> MGNCLDSSAKVDNSNHSPHANSASSGSKVSSKTS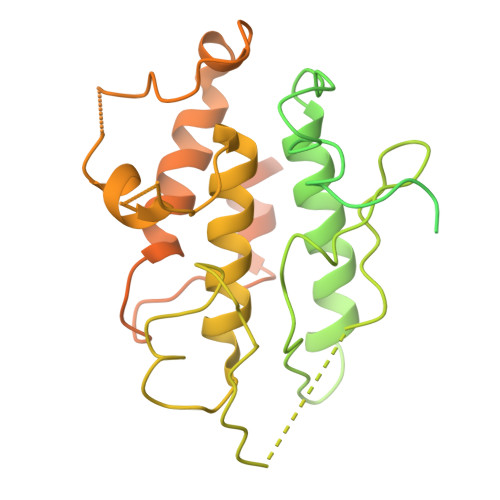RSTGPSGLSTTSYSTDSSFGPLPTLRTEGEILSSPNLKAFTFNELKNATKNFRQDNLLGEGGFGCVFKGWIDQTSLTASRPGSGIVVAVKQLKPEGFQGHKEWLTEVNYLGQLSHPNLVLLVGYCAEGENRLLVYEFMPKGSLENHLFRRGAQPLTWAIRMKVAVGAAKGLTFLHEAKSQVIYRDFKAANILLDADFNAKLSDFGLAKAGPTGDNTHVSTKVIGTHGYAAPEYVATGRLTAKSDVYSFGVVLLELISGRRAMDNSNGGNEYSLVDWATPYLGDKRKLFRIMDTKLGGQYPQKGAFTAANLALQCLNPDAKLRPKMSEVLVTLEQLESVAKPGTKHTQMESPRFHHSSVMQKSPVRYSHDRPLLHMTPGASPLPSYTQSPRVR> ATGTVSLTDVGLDASYAGQVSIGTPAQDFLVIMDSGSSDLWVAGSTCTENFCKQTYTFDTSTSSSFITSSEAFNITYGSGDADGTLGTDTVSMAGFTVSDQTFGVVTSTSANLISYPLSGLMGLAWKSIASSGATPFWQTLAASGDWDSPEMGVYLKRYRGDNTASQIETDGGQILKGGLNTSLYNGSVNYISIDESEKDYWRIPLEAMVIQGNSVSIASSSGGSNPSCAIDTGTTLIGVPSQTANRIYSQIAGAEALSASSGYEGYYQYPCDTEVTVSLQFGGMSYSISNADMNLGSFTRDTSMCTGAFFAMDMSSRSPVQWIVGASFIKNVYTAFRY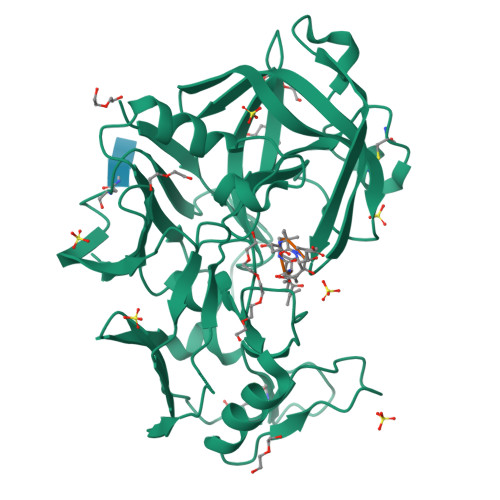NPAAIGFAELV4-{[(2R,5S)-5-{[(2S)-2-(AMINOMETHYL)PYRROLIDIN-1-YL]CARBONYL}PYRROLIDIN-2-YL]METHOXY}-3-TERT-BUTYLBENZOIC 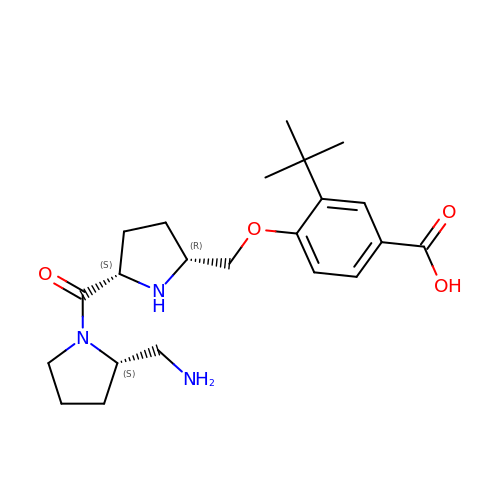ACID | C22 H33 N3 O4 | HSZIDSCIKNQFGX-RYRKJORJSA-N>[2x]RSPWDYKDDDDKLAAANSSIPESWEPCVEVVPNITYQCMELNFYKIPDNLPFSTKNLDLSFNPLRHLGSYSFFSFPELQVLDLSRCEIQTIEDGAYQSLSHLSTLILTGNPIQSLALGAFSGLSSLQKLVAVETNLASLENFPIGHLKTLKELNVAHNLIQSFKLPEYFSNLTNLEHLDLSSNKIQSIYCTDLRVLHQMPLLNLSLDLSLNPMNFIQPGAFKEIRLHKLTLRNNFDSLNVMKTCIQGLAGLEVHRLVLGEFRNEGNLEKFDKSALEGLCNLTIEEFRLAYLDYYLDGIIDLFNCLTNVSSFSLVSVTIERVKDFSYNFGWQHLELVNCKFGQFPTLKLKSLKRLTFTSNKGGNAFSEVDLPSLEFLDLSRNGLSFK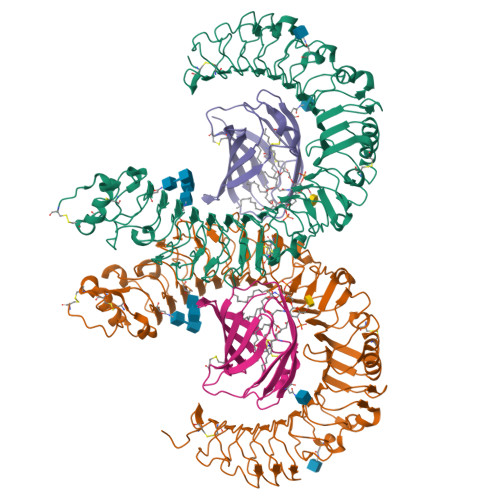GCCSQSDFGTISLKYLDLSFNGVITMSSNFLGLEQLEHLDFQHSNLKQMSEFSVFLSLRNLIYLDISHTHTRVAFNGIFNGLSSLEVLKMAGNSFQENFLPDIFTELRNLTFLDLSQCQLEQLSPTAFNSLSSLQVLNMSHNNFFSLDTFPYKCLNSLQVLDYSLNHIMTSKKQELQHFPSSLAFLNLTQNDFACTCEHQSFLQWIKDQRQLLVEVERMECATPSDKQGMPVLSLNITCQMTGHHHHHH;>EAQKQYWVCNSSDASISYTYCDKMQYPISINVNPCIELKGSKGLLHIFYIPRRDLKQLYFNLYITVNTMNLPKRKEVICRGSDDDYSFCRALKGETVNTTISFSFKGIKFSKGKYKCVVEAISGSPEEMLFCLEFVILHQPNSN[2x]> APAFRYTRSQSFDIFDINQKCFVLESPTQLVALHLQGPSSSQKVRLNIALYRPRGPRGSAGTGQMPVALGIKGYKLYMSCVMSGTEPTLQLEEADVMRDIDSVELTRFIFYR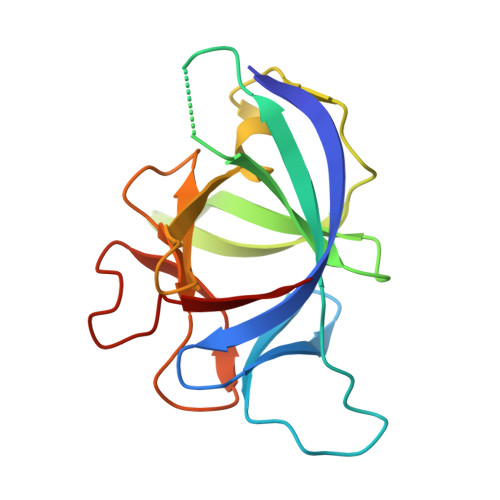LDSPTEGTTRFESAAFPGWFICTSLQPRQPVGITNQPDQVNIATFKLSGR> TVAYIAIGSNLASPLEQVNAALKALGDIPESHILTVSSFYRTPPLG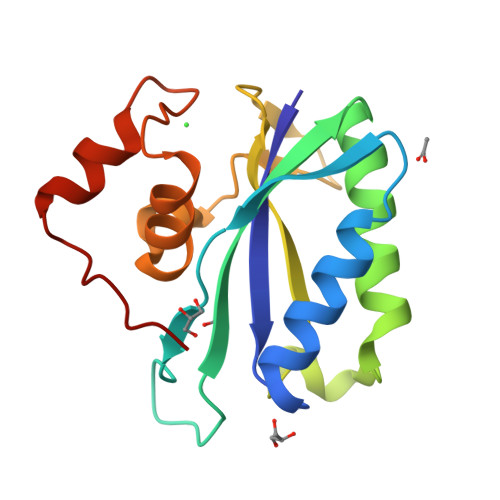PQDQPDALNAAVALETSLAPEELLNHTQRIELQQGRVRKAERWGPRTLDLDIMLFGNEVINTERLTVPHYDMKNRGFMLWPLFEIAPELVFPDGEMLRQILHTRAFDKLNKW> DMPVERILEAELAVEPKTETYVEANMGLNPSSPNDPVTNICQAADKQLFTLVEWAKRIPHFSELPLDDQVILLRAGWNELLIASFSHRSIAVKDGILLATGLHVHRNSAHSAGVGAIFDRVLTELVSKMRDMQM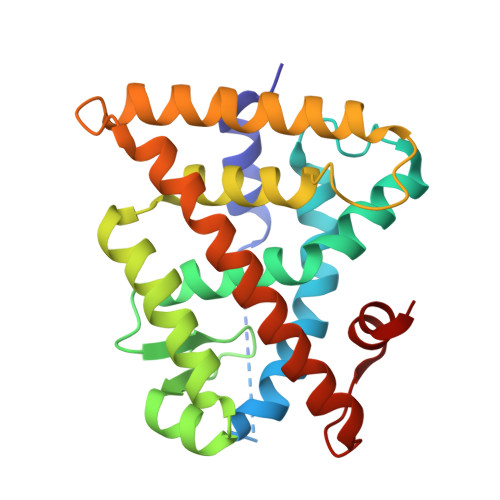DKTELGCLRAIVLFNPDSKGLSNPAEVEALREKVYASLEAYCKHKYPEQPGRFAKLLLRLPALRSIGLKCLEHLFFFKLIGDTPIDTFLMEMLEA>ETGKIFCKSVSKDPDFRLKQIDYVIPVQQDRSICMNNPLLDISDGFFTYIHYEGINSCKKSDSFKVLLSHGEIVDRGDYRPSLYLLSSHYHPYSMQVINCVPVTCNQSSFVFCHISNNTKTLDNSDYSSDEYYITYFNGIDRPKTKKIPINNMTADNRYIHFTFSGGGGVCLGEEFIIPVTTVINTDVFTHDYCESFNCSVQTGKSLKEICSESLRSPTNSSRYNLNGIMIISQNNMTDFKIQLNGITYNKLSFGSPGRLSKTLGQVLYYQSSMSWDTYLKAGFVEKWKPFTPNWMNNTVISRPNQGNCPRYHKCPEICYGGTYNDIAPLDLGKDMYVSVILDSDQLAENPEITVFNSTTILYKERVSKDE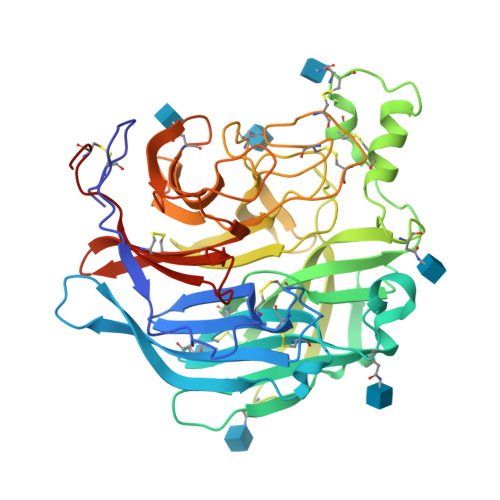LNTRSTTTSCFLFLDEPWCISVLETNRFNGKSIRPEIYSYKIPKYCGTKHHHHHH[2x]>GSHMSAPLPLDELRTFAEVLDRVKAAYVEPVDDKTLLENAIKGMLSNLDPHSAYLGPEDFAELQESTSGEFGGLGIEVGSEDGFIKVVSPIDDTPAARAGIQPGDLIVQIDGKPTKGQSMTEAVDSMRGKAGSPITLTIVRDGGRPFDVELKRAIIKVKSVKSQVLEPGYAYLRITQFQVNTGEEVVKALNQLRKDNKGRLKGLVLDLRNNPGGVLQSAVEVADAFLTKGLIVYTKGRIANSELRFSADPADPSDKVPLVVLING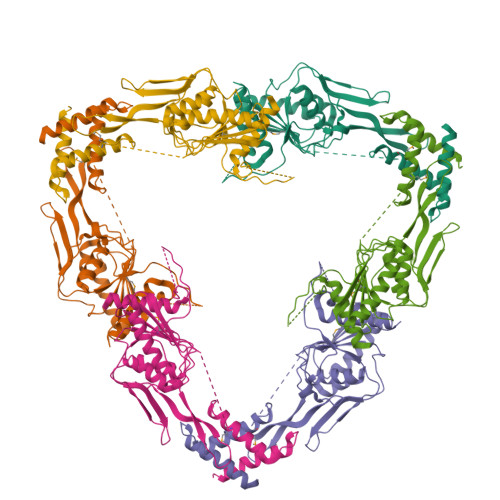GSASAAEIVAGALQDQKRAILMGTDSFGKGSVQTVLPLNNDRALKLTTALYYTPNGRSIQAQGIVPDIEVGRAKVTQERSSFEGFKEADLQGHLANGNGGADRPTGKRAAPSERPQDSDYQLSQALSLLKGLSVTRGN[2x]> AELTKITRGMQNGAETINDNLNKLNTITVQKTGDETIAGKKT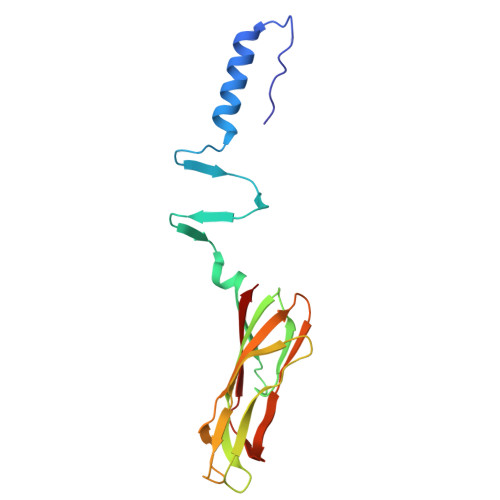FSGDVSVDGDFTMKKFADSYVAFFANKGSGNTVTFTAPWDCTAEVELFYHGWGYSGGEWEIGITTPSGLTQIYEATGYTNGHDNQAISMPTKAIYSGLKKGLQYTFDIRDANGRGGGPKHPMMIVKLYRNA> MSSNNSGLSAAGEIDESLYSRQLYVLGKEAMLKMQTSNVLILGLKGLGVEIAKNVVLAGVKSMTVFDPEPVQLADLSTQFFLTEKDIGQKRGDVTRAKLAELNAYVPVNVLDSLDDVTQLSQFQVVVATDTVSLEDKVKINEFCHSSGIRFISSETRGLFGNTFVDLGDEFTVLDPTGEEPRTGMVSDIEPDGTVTMLDDNRHGLEDGNFVRFSEVEGLDKLNDGTLFKVEVLGPFAFRIGSVKEYGEYKKGGIFTEVKVPRKISFKSLKQQLSNPEFVFSDFAKFDRAAQLHLGFQALHQFAVRHNGELPRTMNDEDANELIKLVTDLSVQQPEVLGEGVDVNEDLIKELSYQARGDIPGVVAFFGGLVAQEVLKACSGKFTPLKQFMYFDSLESLPDPKNFPRNEKTTQPVNSR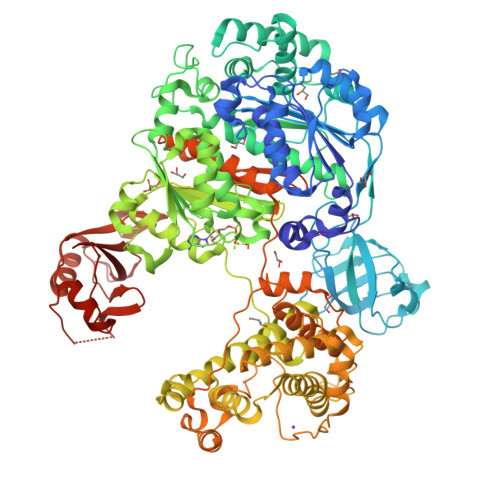YDNQIAVFGLDFQKKIANSKVFLVGSGAIGCEMLKNWALLGLGSGSDGYIVVTDNDSIEKSNLNRQFLFRPKDVGKNKSEVAAEAVCAMNPDLKGKINAKIDKVGPETEEIFNDSFWESLDFVTNALDNVDARTYVDRRCVFYRKPLLESGTLGTKGNTQVIIPRLTESYSSSRDPPEKSIPLCTLRSFPNKIDHTIAWAKSLFQGYFTDSAENVNMYLTQPNFVEQTLKQSGDVKGVLESISDSLSSKPHNFEDCIKWARLEFEKKFNHDIKQLLFNFPKDAKTSNGEPFWSGAKRAPTPLEFDIYNNDHFHFVVAGASLRAYNYGIKSDDSNSKPNVDEYKSVIDHMIIPEFTPNANLKIQVNDDDPDPNANAANGSDEIDQLVSSLPDPSTLAGFKLEPVDFEKDDDTNHHIEFITACSNCRAQNYFIETADRQKTKFIAGRIIPAIATTTSLVTGLVNLELYKLIDNKTDIEQYKNGFVNLALPFFGFSEPIASPKGEYNNKKYDKIWDRFDIKGDIKLSDLIEHFEKDEGLEITMLSYGVSLLYASFFPPKKLKERLNLPITQLVKLVTKKDIPAHVSTMILEICADDKEGEDVEVPFITIHL6-[2-(3'-METHOXYBIPHENYL-3-YL)ETHYL]PYRIDIN-2-AMINE | C20 H20 N2 O | 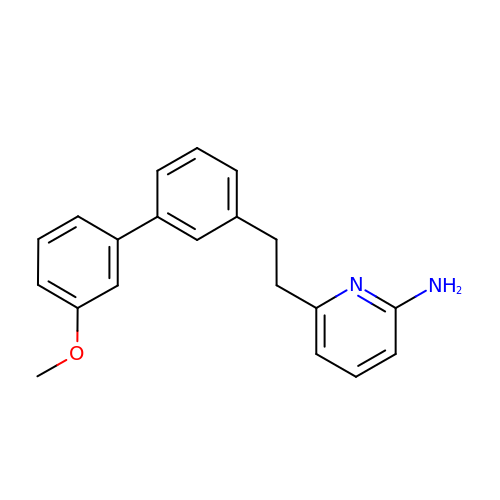AEVBKBAFFJKFJZ-UHFFFAOYSA-N>[2x]GSHMAPEWPMKRDTGCPFDPPPGVRKLLAEKPLSRARIWDGSTPWVVTRHADQRALLSDPRVSHDGLRDGYPHISADFKFLSMAQPSFAGQDDPEHGRIRRMVTLPFTAR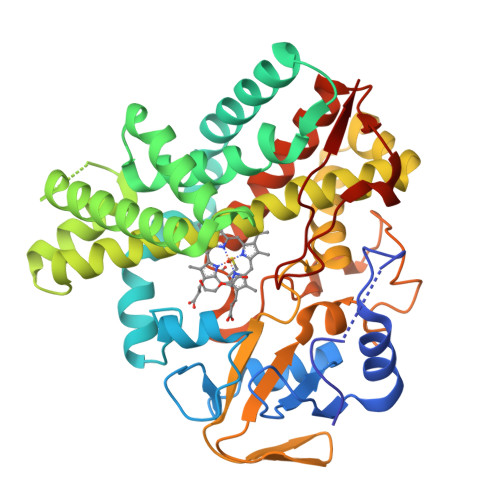RIEAMRPAIQKITDELIDGMLAGPKPVDLVEALALPVPVRVICEMLGVPYEDREFLQQNNNAMIYRDTAQGDAQKAAIAQAMYLKELVGTKLGDRGDDILSDLAVQVEAGEITQDDAAGIGMMLLGAGHETTANMIALGTLALLENPEQLAEVRDSDDPKVIVNTVEELLRYLTIAQDTVRRIAAEDIEIGGVVIKAGEGIVFPLNAANWDPDLYPEAPDRLDIHRANARRHLAFGYGVHQCLGATLARVELQIVYSTLLRRIPTLALAGTLDEIPFKHDQIAHGVYELPVTW>GAMANHLRAEGPASVLAIGTANPENILLQDEFPDYYFRVTKSEHMTQLKEKFRKICDKSMIRKRNCFLNEEHLKQNPRLVEHEMQTLDARQDMLVVEVPKLGKDACAKAIKEWGQPKSKITHLIFTSASTTDMPGADYHCAKLLGLSPSVKRVMMYQLGCYGGGTVLRIAKDIAENNKGARVLAVCCDIMACLFRGPSESDLELLVGQAIFGDGAAAVIVGAEPDESVGERPIFELVSTGQTILPNSEGTIGGHIREAGLIFDLHKDVPMLISNNIEKCLIEAFTPIGISDWNSIFWITHPGGKAILDKVEEKLHLKSDKFVDSRHVLSEHGNMSSSTVLFVMDELRKRSLEEGKSTTGDGFEWGVLFGFGPGLTVERVVVRSVPIKY[3x];> GAMANHLRAEGPASVLAIGTANPENILLQDEFPDYYFRVTKSEHMTQLKEKFRKICDKSMIRKRNCFLNEEHLKQNPRLVEHEMQTLDARQDMLVVEVPKLGAMANHLRAEGPASVLAIGTANPENILLQDEFPDYYFRVTKSEHMTQLKEKFRKICDKSMIRKRNCFLNEEHLKQNPRLVEHEMQTLDARQDMLVVEVPKLGKDACAKAIKEWGQPKSKITHLIFTSASTTDMPGADYHCAKLLGLSPSVKRVMMYQLGCYGGGTVLRIAKDIAENNKGARVLAVCCDIMACLFRGPSESDLELLVGQAIFGDGAAAVIVGAEPDESVGERPIFELVSTGQTILPNSEGTIGGHIREAGLIFDLHKDVPMLISNNIEKCLIEAFTPIGISDWNSIFWITHPGGKAILDKVEEKLHLKSDKFVDSRHVLSEHGNMSSSTVLFVMDELRKRSLEEGKSTTGDGFEWGVLFGFGPGLTVERVVV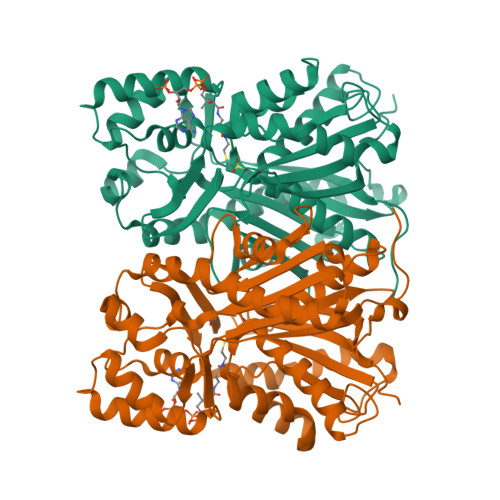RSVPIKY>[2x]MHTQVHTARL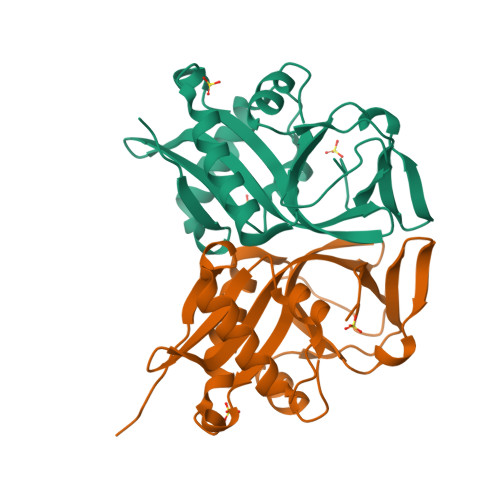VHTADLDSETRQDIRQMVTGAFAGDFTETDWEHTLGGMHALIWHHGAIIAHAAVIQRRLIYRGNALRCGYVEGVAVRADWRGQRLVSALLDAVEQVMRGAYQLGALSSSARARRLYASRGWLPWHGPTSVLAPTGPVRTPDDDGTVFVLPIDISLDTSAELMCDWRAGDVW>[2x]ANRTLIVTTILEEPYVMYRKSDKPLYGNDRFEGYCLDLLKELSNILGFIYDVKLVPDGKYGAQNDKGEWNGMVKELIDHRADLAVAPLTITYVREKVIDFSKPFMTL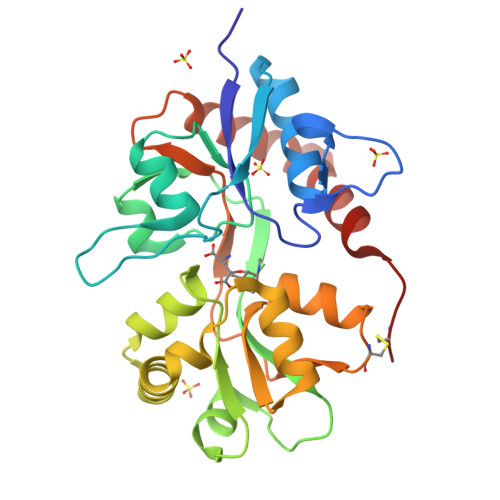GISILYRKGTPIDSADDLAKQTKIEYGAVRDGSTMTFFKKSKISTYEKMWAFMSSRQQTALVRNSDEGIQRVLTTDYALLMESTSIEYVTQRNCNLTQIGGLIDSKGYGVGTPIGSPYRDKITIAILQLQEEGKLHMMKEKWWRGNGCP>HMNEHNLLIFCLKDNVSISEYTEMIDWAYKNIQSETVVEITENQIIEYQNRGLWRLVSEITDNWLFGPSEGDWLIDKESILAVKEKLQNSDFSTEPLVKNIIHVLEYAIK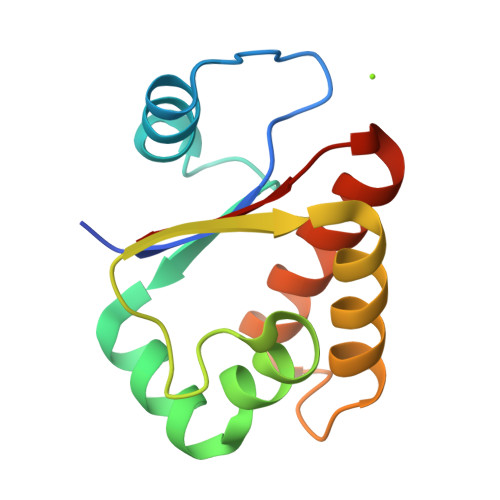NEKTVIFHF[2x]(3R)-3-[(7-{[(2S)-2-amino-2-(2-methoxyphenyl)ethyl]amino}-5-methyl[1,2,4]triazolo[1,5-a]pyrimidin-2-yl)amino]-3-(3-chlorophenyl)propanenitrile | C24 H25 Cl N8 O 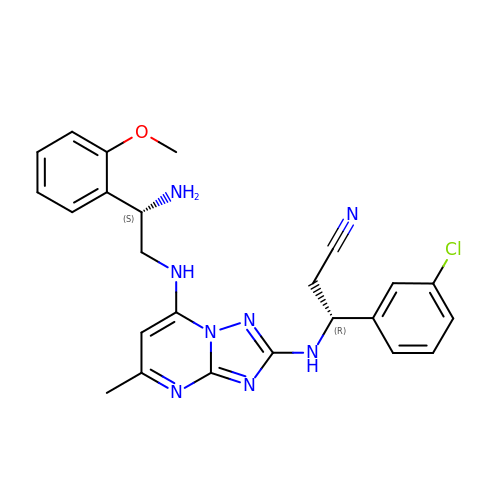| TVYFBBBTUXLKKX-WOJBJXKFSA-N> MAHHHHHHMAIRKILYLPDERLRKIAKPVETFDESLQTLINDMFDTMYDARGVGLAAPQIGVSLRLSVIDIVGDKKEQIVIVNPEIVSSHGEKEFEEGCLSVPGAYDTVVRAEKVTVKALDRFGKPFEITGEG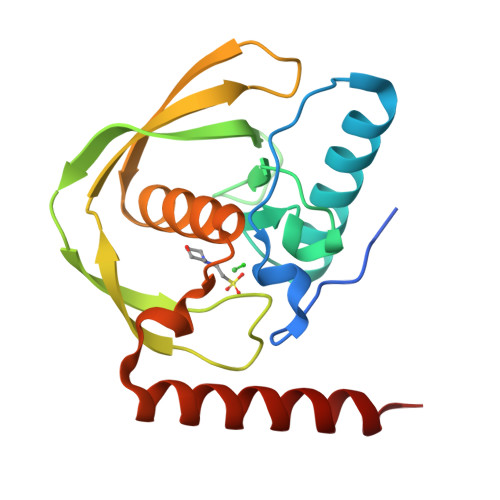LLAECLQHEIDHMNGKLFVDMLSPLKRMMARRKLDKFKRLQARKP> MKRARPSEDTFNPV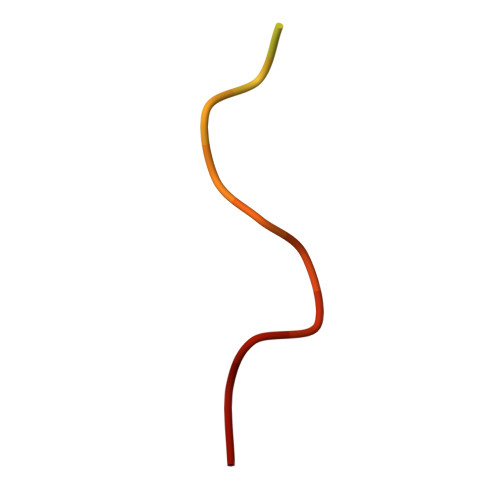YPYDTEC>MNTQILVFALIAIIPTNADKISAWSHPQFEKGGGGSHHHHHHSSSGSGAHIVMVDAYKPTKGGSGGGGSIINETADDIVYRLTVIIDDRYESLKNLITLRADRLEMIINDNVSTILAGGSGTGSVTLAGNSSLCPISGWAIYSKDNGIRIGSKGDVFVIREPFISCSHLECRTFFLTQGALLNDKHSNGTIKDRSPYRTLMSCPVGEAPSPYNSRFESVAWSASACHDGISWLTIGISGPDNGAVAVVKYNGIITDTIKSWRNKILRTQESECACVNGSCFTVMTDGPSDGQASYKIFKIEKGKVVKSVEMKAPNYHYEECSCYPDAGDIMCVCRDNWHGSNRPWVSFNQNLEYQMGYICSGVFGDNPRPNDKTGSCGPVSSNGANGVKGFSFKYGNGVWIGRTKSISSRKGFEMIWDPNGWTETDSSFSVKQDIVGINEWSGYSGSFVQHPEMTGLDCMRPCFWVELIRGRPEENTIWTSGSSISFCGVNSDTVGWSWPDGAELPFTIDK[2x]

Influenza virus neuraminidase (NA) is an important target for protective antibodies and therapeutic drugs against influenza viruses. NA cleaves off host sialic acids, aiding the release of newly formed virions from infected cells. NA is a mushroom-shaped type II homotetrameric protein. The polypeptide chain of the NA monomeric head folds into six, topologically identical, four-stranded, antiparallel β-sheets which are arranged like the blades of a propeller.

N1/19 hybrid means loops 01 and 23 of N1/2019 grafted to mSN1 (H5N1/2021) scaffold. Similarly, 16 dissimilar residues within Loops 01 and 23 of N1/19 were transferred to mS N1 scaffold to form N1/19 hybrid. The N1/09 hybrid showed an 8°C improvement in its melting temperature Tm to 64.4°C compared to the N1/09 protein (56.4°C), while the Tm of the N1/19 hybrid (72.4°C) surpassed the H5N1 mSN1 scaffold donor (68.7°C). The CD6 epitope was lost on seasonal H1N1 viruses isolated after 2015 (unpublished observation) so CD6 bound to cells infected with N1/09 but not N1/19 virus, but CD6 bound to the N1/19 hybrid protein strongly, suggesting that CD6’s binding to the N1/19 hybrid depended on the scaffold residues donated by the msN1 protein, and that the N1/19 hybrid protein had formed a compact tetramer compatible with the N1/19 hybrid’s higher Tm of 72.4°C. Similarly, NmAb-03, displaying specific binding to N1/19 NA on infected cells, exclusively bound to the N1/19 hybrid protein. To assess whether loop grafting influenced the local or overall structure of the NA, we determined high resolution crystal structures of mSN1, the N1/09 hybrid, and the N1/19 hybrid. Overlay analysis revealed that N1/09 hybrid and N1/19 hybrid were nearly identical in structure to mSN1, with overall RMSDs of <0.25 Å across equivalent Cα atoms upon overlay (Meng et al., 2023). In contrast, the N1/09 and N1/19 hybrids show no noticeable differences between the protomer cavities, all of which closely resemble the wider msN1(ii) conformation, apart from minor, local widening of the rim induced by the substitution of Y344 with an asparagine residue (shown as light-green sticks). Additionally, we observed that the Y344N substitution in the N1/09 and N1/19 hybrids slightly widened the enzymatic cavity compared to msN1. The mSN1 and the N1/19 hybrid both induced strong inhibitory antibodies to themselves, but the sera to mSN1 failed to cross-inhibit the enzyme activity of N1/19-like virus and the N1/19 hybrid protein did not generate a cross-inhibitory NAI antibody response to mSN1.> MQQGQMAYDRAITVFSPDGRLFQVEYA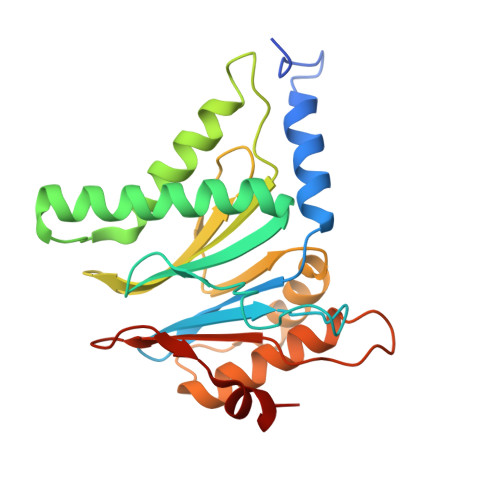REAVKKGSTALGMKFANGVLLISDKKVRSRLIEQNSIEKIQLIDDYVAAVTSGLVADARVLVDFARISAQQEKVTYGSLVNIENLVKRVADQMQQYTQYGGVRPYGVSLIFAGIDQIGPRLFDCDPAGTINEYKATAIGSGKDAVVSFLEREYKENLPEKEAVTLGIKALKSSLEEGEELKAPEIASITVGNKYRIYDQEEVKKFL2-amino-7,7-dimethyl-5,6,7,8-tetrahydro-4H-[1,3]thiazolo[5,4-c]azepin-4-one | C9 H13 N3 O S | 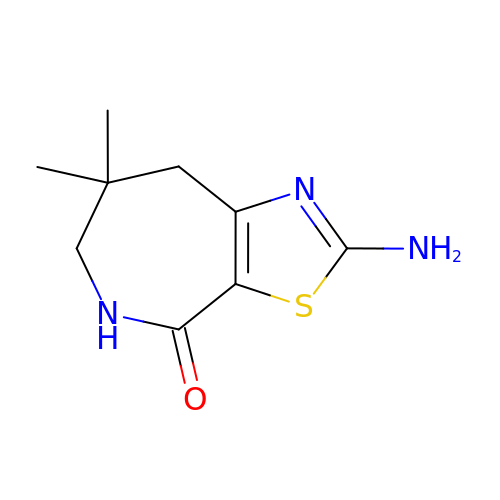KRPZAWRISMXVDQ-UHFFFAOYSA-N> MARHGKGPKTNKKKLAPEKERFIQCCADITLELTDSLTSGTTREINLNGLITKYSKKYKLKQQPRLTDIINSIPDQYKKYLLPKLKAKPVRTASGIAVVAVMCKPHRCPHIAYTGNICVYCPGGPDSDFEYSTQSYTGYEPTSMRAIRARYDPYEQARGRVEQLKQLGHSIDKVEYVLMGGTFMSLPKEYREDFIVKLHNALSGFNGNDIDEAILYSQQSLTKCVGITIETRPDYCTQTHLDDMLKYGCTRLEIGVQSLYEDVARDTNRGHTVRSVCETFAVSKDAGYKVVSHMMPDLPNVGMERDIEQFKEYFENPDFRTDGLKIYPTLVIRGTGLYELWKTGRYKSYSANALVDLVARILALVPPWTRIYRVQRDIPMPLVTSGVDNGNLRELALARMKDLGTTCRDVRTREVGIQEVHHKVQPDQVELIR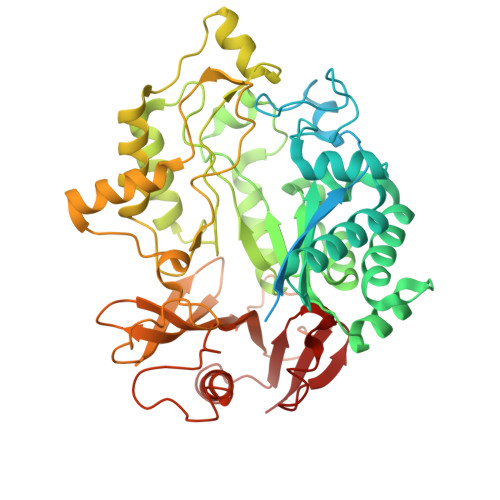RDYYANGGWETFLSYEDPKKDILIGLLRLRKASKKYTYRKEFTSQRTSIVRELHVYGSVVPLHSRDPRKFQHQGFGTLLMEEAERIAKEEHGSEKISVISGVGVRNYYGKLGYELDGPYMSKRI>SQARVSDVEEQVNQYLSKVPELEQKQNVSELLSLLSNSPNISLSQLKAYLEGKSEEPSEQFKMLCGLRDALKGRPELAHLSHLVEQALVSMAEEQGETIVLGARITPEAYRESQSGVNPLQPLRDTYRDAVMGYQGIYAIWSDLQKRFPNGDIDSVILFLQKALSADLQSQQSGSGREKLGIVISDLQKLKEFGSVSDQVKGFWQFFSEGKTNGVRPF[2x];>[2x]MAYDLSEFMGDIVALVDKRWAGIHDIEHLANAF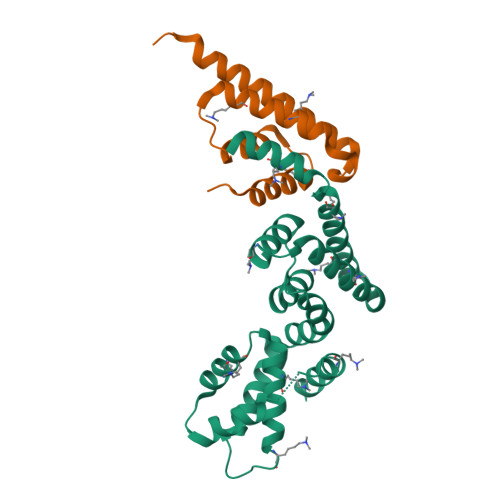SLPTPEIKVRFYQDLKRMFRLFPLGVFSDEEQRQNLLQMCQNAIDMAIESEEEELSELD> MHLPNGAQIFVETSRGEEIEATAVTNEKNPVATVASKGDLAKGDYVIVTQSTWAKMVSRVLIVTDAQETSITLAGIDTSDTLVFPAGGTMSFAKITGWTEIPCVQEIGQDGGEQQYYTYQCLSDDKEQQIPTFKSAISLTYTFAHEFDNPIYQILRKLDSSGQVTAVRMYVPKASEMRMWAGILSFNDIPSTQVNEMET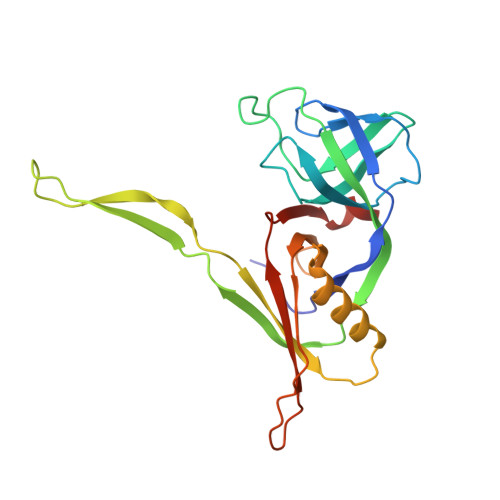VELAVSLKGDFTFISSTLASPGA> MSFINYSSREINCKIVYYGPGLCGKTTNLQYIYNKTAAETKGKLISLSTETDRTLFFDFLPLSLGEIRGFKTRFHLYTVPGQVFYDASRKLILKGVDGVVFVADSQIERM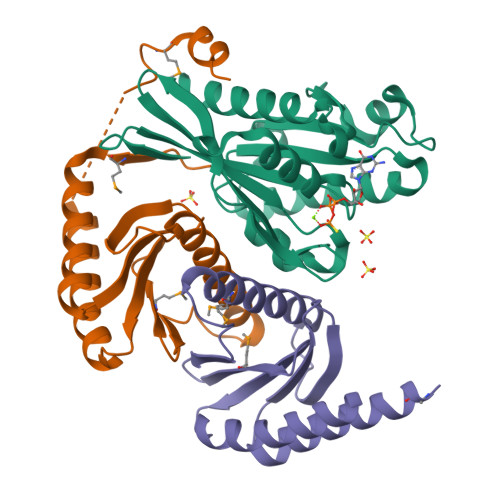EANMESLENLRINLAEQGYDLNKIPYVIQYNKRDLPNAVTVEEMRKALNHRNIPEYQAVAPTGVGVFDTLKAVAKLVLTELKKGGGSHHHHHH;>MGTQLVMYEEEFTKINAVCDRLTKDANAKVVFLVDKNGQLISSAGQTQNIDTTSLASLTAGNVAAMGGLAKLIGENEFPNQFHEGAKDSLYMTIVGSRVVLVVIFDNRTSLGLVRLRIKKASDELTKIFESLVKKTDSPGAGSPFAEMSDDDIDNLFSEGSHHHHHH[2x]>MHHHHHHGGLVPRGSHMKIGIIGAMEEEVTLLRDKIDNRQTITLGGCEIYTGQLNGTEVALLKSGIGKVAAALGATLLLEHCKPDVIINTGSAGGLASTLKVGDIVVSDETRYHDADVTAFGYEYGQL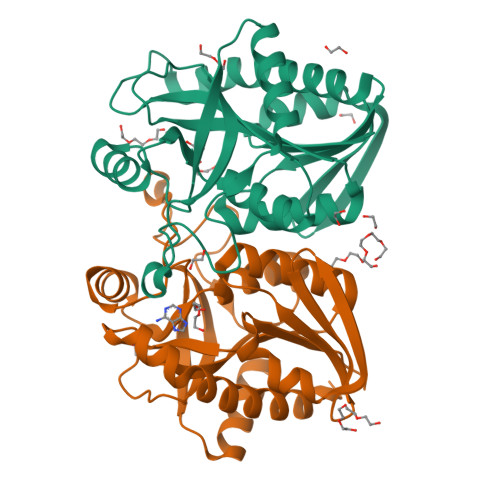PGCPAGFKADDKLIAAAESCIRELNLNAVRGLIVSGDAFINGSVGLAKIRHNFPDAVAVEMEATAIAHVCHNFNVPFVVVRAISDVADQQSHLSFDEFLAVAAKQSTLMVETLVQKLAHG[2x]>MQLERRKRGTMEIMFDILRNCEPKCGITRVIYGAGINYVVAQKYLDQLVKVGALNIKTENDRKIYEITEKGKLLRTHIEEFIKIRENLYSAKEKVSELLRTDSE[3x]

Three Sso10a homologues are encoded on the S. solfataricus genome: Sso10a1, Sso10a2 and Sso10a3 (29–39% sequence identity and 55–62% sequence similarity). The structure of Sso10a1 reveals that it dimerises in solution via the formation of an anti-parallel coiled-coil structure16. The domain at the end of the coiled-coil is believed to be involved in DNA-binding as it adopts a winged helix-turn-helix (wHTH) motif. Based on our findings we conclude that the Sso10a proteins function as chromatin proteins; they bind DNA with high affinity, and display different architectural properties (DNA bending, bridging and stiffening).

Dimerization occurs through an anti-parallel coiled-coil interaction of the α4-helix. A notable difference in the amino acid sequence of the three Sso10a proteins is that Sso10a2 contains four extra residues within the winged loop domain, not present in Sso10a1 and Sso10a3. The four extra amino acids at position 56–59 in Sso10a2 lead to an extended loop within the wing domain. Sso10a1 and Sso10a2 structures also differ in the orientation angle between the α3-helices. As the relative position and orientation of the two α3-helices is predicted to have an important influence on the DNA-binding mode, this could result in distinctly different DNA-binding properties for Sso10a1 and Sso10a2. Note that the Sso10a2 crystal structure suggests possible electrostatic interactions (K57-E59 and E59-K57) between the wings of adjacent dimers. Such interactions could underlie the observed DNA stiffening and the salt sensitivity of this process (see Discussion & Conclusions). The increase of RMS at high concentrations of Sso10a2 suggests that, besides bending and/or bridging, Sso10a2 has a second binding mode which leads to the formation of stiff protein-DNA filaments. The effect of NaCl concentration on the stiffening mode suggests that this binding mode is determined by electrostatic interactions between neighboring proteins.> SLTFYPAWLTVSEGANATFTCSLSNWSEDLMLNWNRLSPSNQTEKQAAFSNGLSQPVQDARFQIIQLPNRHDFHMNILDTRRNDSGIYLCGA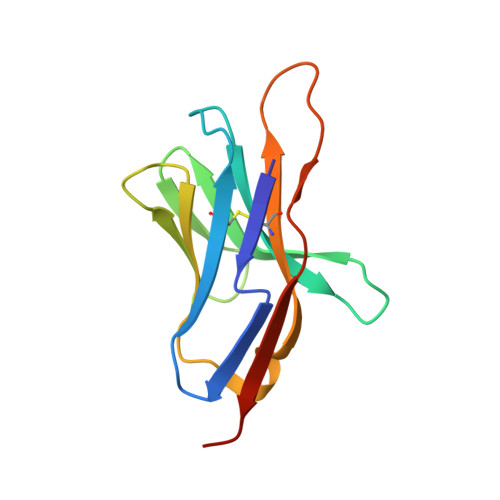ISLHPKAKIEESPGAELVVTERILE>[2x]GAGAGAGAGAGMGQPTTTSLFMRDVMFHRMTGTSQAVNDVATLSGERREIIRRALNKKILVPNILELMPAWPSEFQPNIDEVNVEIDEWLKTVNVAKEKKLKHRARGNYTLLAGIYYPHCRKEKMLALSQFLYWIFFWDDEIDTGGELTEDREGTILCCAETNKCINDCLGPEPNY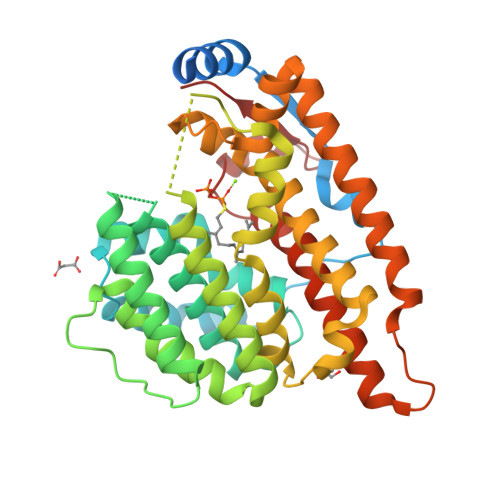TPPPGSRGTVEMLYPILRDLRAGLSPVSTMRLKQELHDYVNGVKNQQKVRQEDHLPNPWDHFQMRVDDVGVIPSITQNEYAMDFTLPDWIRRHEAMEEIVLQCTKLTILLNEILSLQKEFRVSQLENLCLLFMNTYDMSIEQSIHKVLGLLKDHYKICIEAEARLPWSTTDEKLNNNIREYIRGCQRLATGTACWSYNCERYFKLSQLNDQQELLLDLSRT>[2x]SSLPLNAIEPCVICQGRPKNGCIVHGKTGHLMACFTCAKKLKKRNKPCPVCRQPIQMIVLTYFP;>[2x]EDCQNLLKPCSLCEKRPRDGNIIHGRTGHLVTCF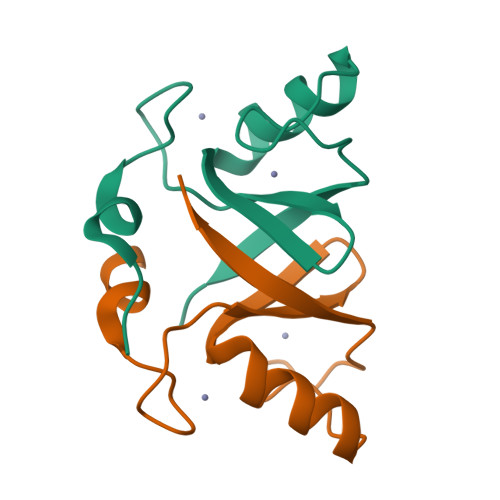HCARRLKKAGASCPICKKEIQLVIKVFIA(4S,5R)-4,5-dihydroxy-5-[(3E,6E)-octa-3,6-dien-1-yl]pyrrolidin-2-one | C12 H19 N 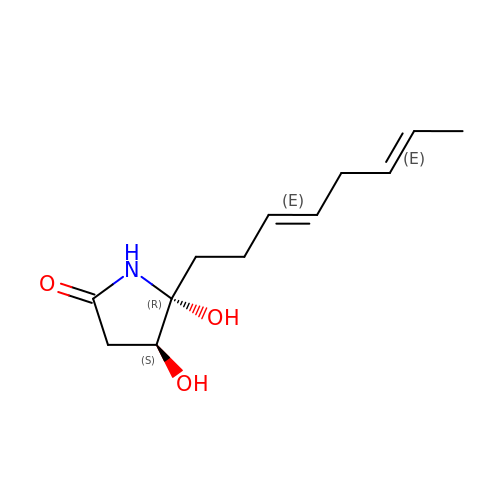O3 | VIMHNMLESUAQPL-JFDNTZKISA-N> GSLTYAQAQGMVEIEIEGRLHRISIFDPLEIILED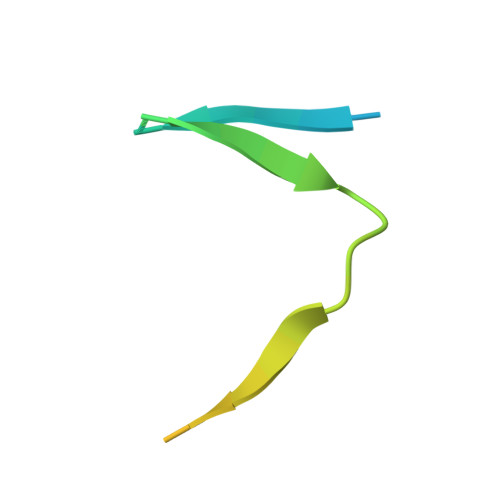DLTAQEMSECNSNKENS>[2x]NENSDVSRAEEFKSQANEAFKGHKYSSAIDLYTKAIELNSNNAVYWANRAFAHTKLEEYGSAIQDASKAIEVDSRYSKGYYRRGAAYLAMGKFKDALKDFQQVKRLSPNDPDATRKLKECEKAVMKLKFEEAISVPVSERRSVAESIDFHTIEVEPQYSGARIEGEEVTLDFVKTMMEDFKNQKTLHKRYAYQ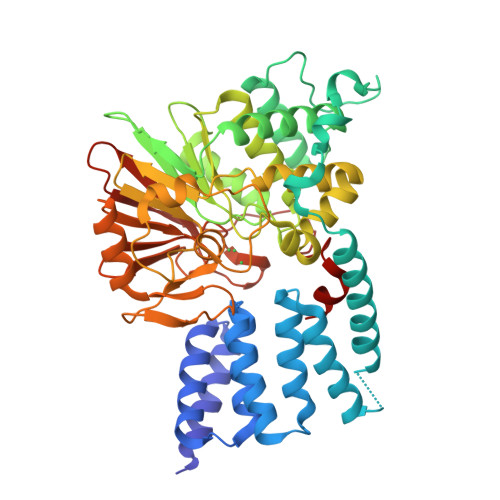IVLQTRQILLALPSLVDISVPHGKHITVCGDVHGQFYDLLNIFELNGLPSEENPYLFNGDFVDRGSFSVEIILTLFAFKCMCPSSIYLARGNHESKSMNKIYGFEGEVRSKLSEKFVDLFAEVFCYLPLAHVINGKVFVVHGGLFSVDGVKLSDIRAIDRFCEPPEEGLMCELLWSDPQPLPGRGPSKRGVGLSFGGDVTKRFLQDNNLDLLVRSHEVKDEGYEVEHDGKLITVFSAPNYCDQMGNKGAFIRFEAPDMKPNIVTFSAVPHPDVKPMAYANNFLRMF> DNSRYTHFLTQHYDAKPQGRDDRYCESIMRRRGLTSPCKDINTFIHGNKRSIKAICENKNGNPHRENL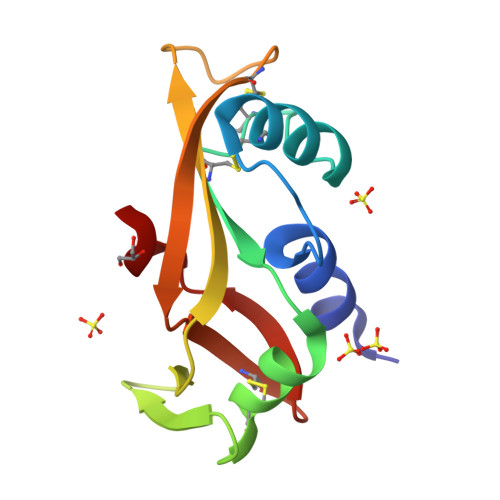RISKSSFQVTTCKLHGGSPWPPCQYRATAGFRNVVVACENGLPVHLDQSIFR> MKEIKLMADYHCYPLWGTTPDDFGDISPDELPISLGLKNSLEAWAKRYDAILNTDDPALSGFKSVEEEKL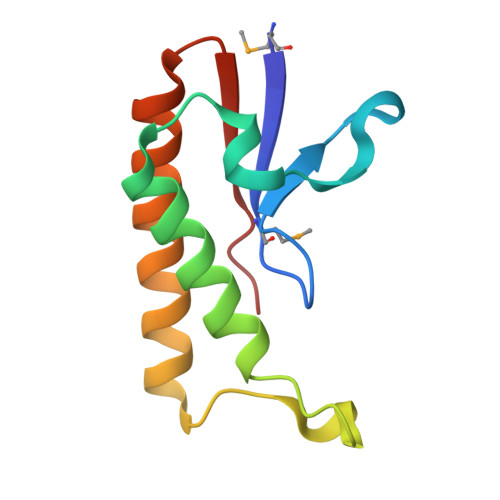FIDDGYKLAELLQEELGSAYKVIYHADY>[3x]MSTNKVNKERTFLAVKPDGVARGLVGEIIARYEKKGFVLVGLKQLVPTKDLAESHYAEHKERPFFGGLVS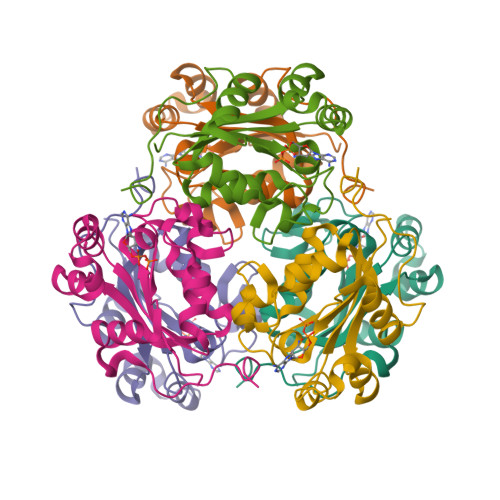FITSGPVVAMVFEGKGVVASARLMIGVTNPLASAPGSIRGDFGVDVGRNIIHGSDSVESANREIALWFKPEELLTEVKPNPNLYE>[12x]MIVRTQNSESKIKEFFEFCKENEVEFVDFRFSDIKGTWNHIAYSFGALTHGMLKEGIPFDASCFKGWQGIEHSDMILTPDLVRYFIDPFSADVSVVVFCDVYDVYKNQPYEKCPRSIAKKALQHLKDSGLGDVAYFGAENEFFIFDSIKIKDASNSQYYEVDSEEGEWNRDRSF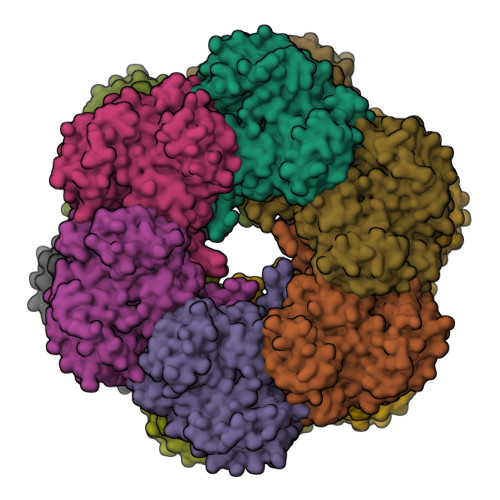ENGVNFGHRPGKQGGYMPVPPTDTMMDIRTEIVKVLNQVGLETFVVHHEVAQAQGEVGVKFGDLVEAADNVQKLKYVVKMVAHLNGKTATFMPKPLYGDNGSGMHTHVSVWKNNENLFSGETYKGLSEFALHFLGGVLRHARGLAAFTNASTNSYKRLIPGYEAPSILTYSANNRSASVRIPYGISKNSARFEFRFPDSSSNPYLAFAAILMAGMDGVKNKIDPGEAMDINLFKLTLDEIREKGIKQMPHTLRRSLEEMLADKQYLKESQVFSEEFIQAYQSLKFNAEVFPWESKPHPFEFITTYSC> SDHHHHHHGPISPIETVPVKLKPGMDGPKVKQWPLTEEKIKALVEICTEMEKEGKISKIGPENPYNTPVFAIKKKDSTKWRKLVDFRELNKRTQDFWEVQLGIPHPAGLKKKKSVTVLDVGDAYFSVPLDEDFRKYTAFTIPSINNETPGIRYQYNVLPQGWKG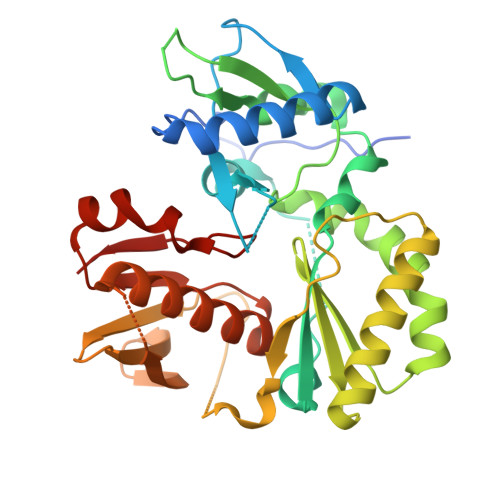SPAIFQSSMTKILEPFKKQNPDIVIYQYMDDLYVGSDLEIGQHRTKIEELRQHLLRWGLEPPFLWMGYELHPDKWTGSGSGGYDPSKDLIAEIQKQGQGQWTYQIYQEPSKNLKTGKYARKRGAHTNDVKQLTEAVQKITTESIVIWGKTPKFKLPIQKETWETWWTEYWQATWIPEWEFVN Recent research has identified the Mpr1/Pad1 N-terminal (MPN) domain-containing protein (MPND) as a sensor protein that may recognize DNA 6mA modification in eukaryotes. Moreover, the Mpr1/Pad1 N-terminal (MPN) domain-containing protein (MPND) was the first reported protein containing the RAMA domain to directly bind to DNA with the 6mA modification in vitro. In this work, we investigated the first crystal structures of the apo–MPND and the MPND–DNA complex from Mus musculus at the atomic resolution. Our results revealed that MPND possesses multiple functions, such as binding DNA and interacting with histones.

We used different MPND truncations with dsDNA to generate stable complexes for crystal screening and, fortunately, obtained the complex crystal for the fragment (residues 54–163). The complex was refined to 2.47 Å in the space group P1, with an Rwork of 24.5% and an Rfree of 25.4%. The final refined complex structure contained four MPND molecules, as well as one dsDNA in the asymmetric unit. However, as the DNA recognition by MPND appeared to be sequence-independent, and the DNA bases were averaged in the structure determination, the final nucleic acid density could only correspond to 10 base pairs. Therefore, we modeled the adenine and thymine into the electron density. Among the four MPND molecules solved in the asymmetric unit, only two MPND molecules were involved in direct contact with dsDNA. The primary protein–DNA interactions between MPND and dsDNA were the hydrogen bonds formed between Ser113, Ser115, Trp135, and the DNA backbone. However, no specific protein–base interaction was found. When compared with the apo–MPND structure, the orientation of the N-terminal loop changed upon binding to dsDNA, and R63 moved over the major groove of dsDNA. The overall conformation of MPND between the apo- and DNA-bound forms was found to be similar, as demonstrated by the structural superposition, with the RMSD of all Cα atoms being just 0.8 Å.

>GSAAPESLSPGATAEEAPEEDEDDAEAEDPERGTGSGGRSGSLGGSGGGTAGPGMALGGALTRRAVTLRVLLKDELLEPGEGVLSIYYLGRKFTGDLQLDGRIVWQETGQVFNSPSAWATHCKKLVNPAKKSGCGWASVKYKGQKLDKYKAAWLRRHQLHM[4x]> MNFNVSLMEKLKWKIKCIENKFLNYRLTTNETVVAETEYGKVKGVKRLTVYDDSYYSFEGIPYAQPPVGELRFKAPQRPTPWDGVRDCCNHKDKSVQVDFIAGKVCGSEDCLYLSVYTNNLNPETKRPVLVYIHGGDFIIGENHRDMYGPDYFIKKDVVLINIQYRLGALGFLSLNSEDLNVPGNAGLKDQVMALRWIKNNCANFGGNPDNITVFGESAGAASTHYMMLTEQTRGLFHRGILMSGNAICPWANTQCQHRAFALAKLAGYKGEDNDKDVLEFLMKAKPQDLIKLEEKVLTLEERTNMVVFPFGPTVEPYQTADCVLPKHPREMVKTAWGNSIPTMMGNTSYEGLFFTSILKQMPMLVKELETCVNFVPSELADAERTAPETLEMGAKIKKAHVTGETPTADNFMDLCSHIYFWFPMHRLLQLRFNHTSGTPVYLYRFDFDSEDLINPYRIMRSGRGVKGVSHADELSYFFWNQLAKRMPKESREYKTIERMTGIWIQFATTGNPYSNEIEGMENVSWDPIKKSDEVYKCLNISDELKMIDVPEMDKIKQWESMFE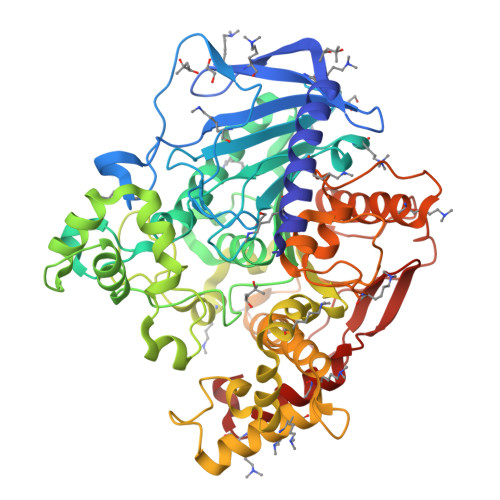KHRDLF> MKKGHHH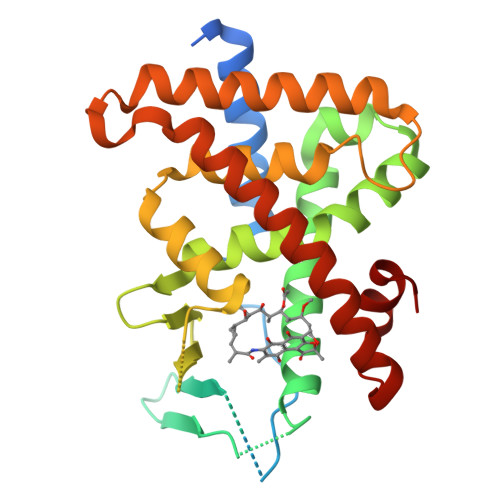HHHGSERTGTQPLGVQGLTEEQRMMIRELMDAQMKTFDTTFSHFKNFRLPGVLSSGCELPESLQAPSREEAAKWSQVRKDLCSLKVSLQLRGEDGSVWNYKPPADSGGKEIFSLLPHMADMSTYMFKGIISFAKVISYFRDLPIEDQISLLKGAAFELCQLRFNTVFNAETGTWECGRLSYCLEDTAGGFQQLLLEPMLKFHYMLKKLQLHEEEYVLMQAISLFSPDRPGVLQHRVVDQLQEQFAITLKSYIECNRPQPAHRFLFLKIMAMLTELRSINAQHTQRLLRIQDIHPFATPLMQELFGI> SLEDYSVVNRFESHGGGWGYSAHSVEAIRFSADTDILLGGLGLFGGRGEYTAKIKLFELGPDGGDHETDGDLLAETDVLAYDCAAREKYAMMFDEPVLLQAGWWYVAWARVSGPSSDCGSHGQASITTDDGVIFQFKSSKKSNNGTDVNAGQIPQL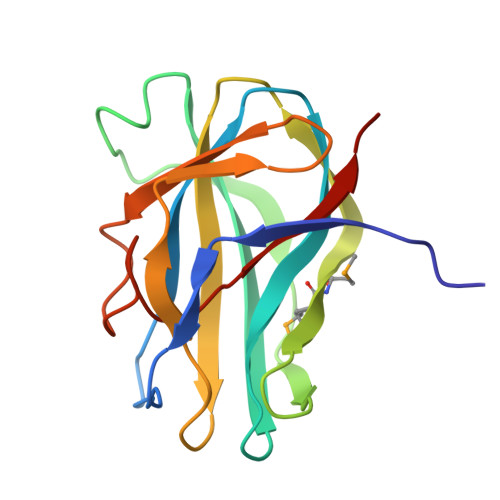LYRLPTSD> GHMQRIRIIDSHTGGEPTRLVIGGFPDLGQGDMAERRRLLGERHDAWRAACILEPRGSDVLVGALLCAPVDPEACAGVIFFNNSGYLGMCGHGTIGLVASL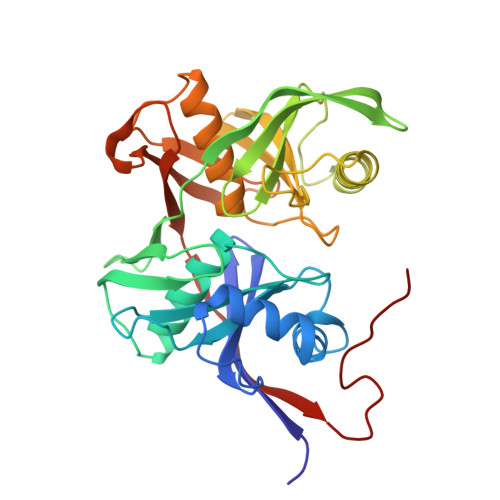AHLGRIGPGVHRIETPVGEVEATLHEDGSVSVRNVPAYRYRRQVSVEVPGIGRVSGDIAWGGNWFFLVAGHGQRLAGDNLDALTAYTVAVQQALDDQDIRGEDGGAIDHIELFADDPHADSRNFVLCPGKAYDRSPCGTGTSAKLACLAADGKLLPGQPWRQASVIGSQFEGRYEWLDGQPGGPIVPTIRGRAHVSAEATLLLADDDPFAWGIRRGS4-(2-azanylethoxy)phenol 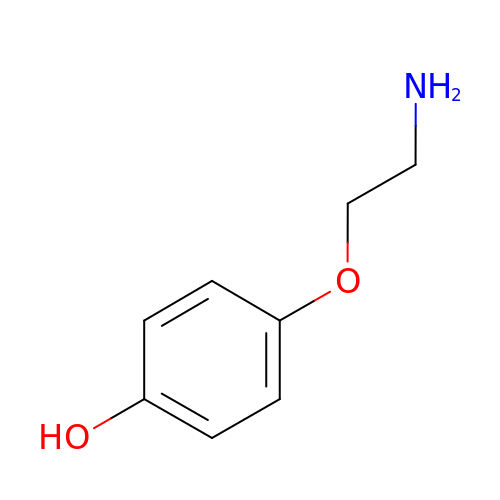| C8 H11 N O2 | QSDOKFGRSJQNMX-UHFFFAOYSA-N> MESKNKTAATQQSEPNVIAAHKGVNQAPVPLKMERVGPHDVHIEMTAQITDIEIDKGKIYKAWTFNGQAPGPLVVVNEGDTIHFTLKNMDPVVPHSMDFHAVHASPSKDFIDVMPNKSGTFTYPANKPGVFMYHAGTKPVLQHIANGMHGVIIVKPKNGYPTDKEVDREYVLIQNEWYKYNDMNDFQNGVPSYVVFSSKALKPGDPNTNGDTFTLKEKPLLAKVGEKIRLYINNVGPNEVSSFHVVGTVFDDVYLDGNPNNHLQGMQTVMLPASGGAVVEFTVTRPGTYPIVTHQFNHAQKGAVAMLKVTETGEDDGTETSGH

Copper-containing nitrite reductases (CuNIRs) catalyze transformation of nitrite to nitric oxide, which has impacts on geochemical, agricultural, and medical health fields. CuNIRs typically have an ∼110 kDa homotrimeric structure, like a Reuleaux triangle. Each protomer contains one type 1 copper (T1Cu) and one type 2 copper (T2Cu) site. The Cys residue forms a peptide-bond bridge (Cys-His bridge) together with one of the His ligands at the T2Cu site to transfer the electron to the catalytic T2Cu site, which is coordinated by three His residues and an axial water molecule.

We bypassed the problem that NO2- decomposes during RT neutron data collection by using formic acid, a stable analog of NO2- and an inhibitor of NO2- reduction. RT ND and XRD data up to 1.90 and 1.20 Å resolution, respectively, were collected from a single crystal of C135A GtNIR in complex with deuterated formic acid and we determined the structure. The electron density shows that formate binds to the T2Cu atom, although it has low occupancy (0.54). The D atom on the central C atom of formate cannot be visualized in the neutron-scattering length density map although the omit map implies its presence, indicating that the formate ligand is unstable and its position at the T2Cu site fluctuates. Formate assumes a κ1-O mode, which is observed in a previously reported cryogenic structure. This finding suggests that differences of data collection temperature do not affect the binding mode of indecomposable ligands. Therefore, the difference of the NO2- binding manners is probably caused by X-ray photoreduction that is greatly facilitated at higher temperatures. OH- is present on one of the two axial sites of the T2Cu in the resting and NO2--bound states, but is partially replaced by a water molecule in the formate-bound structure. This finding means that the ligand at this position can easily absorb and desorb H+ at RT and interconvert between OH- and H2O.The family Iflaviridae of insect viruses includes important pathogens of the western honeybee (Apis mellifera): deformed wing virus (DWV), sacbrood virus (SBV), and slow bee paralysis virus (SBPV). The icosahedral capsids of iflaviruses protect single-stranded RNA genomes that are about 10,000 nucleotides long and are polyadenylated at the 3′ end. Capsid proteins VP1, VP2, and VP0, originating from one polyprotein, form a protomer, 60 of which assemble into a pseudo-T = 3 icosahedral capsid. Subunits VP3 of DWV and SBPV have 160-residue-long C-terminal extensions, which fold into globular domains protruding from the virion surface.

The genome release of iflaviruses can be induced in vitro by exposing the particles to acidic pH. We show that acidic pH induces expansion of the RNA genome in the DWV particle, which, in turn, triggers the swelling and flower-like opening of its capsid. Native virions of DWV at neutral pH are uniform in size with a radius (the distance of the center of the mass of a pentamer from the center of the capsid) of 135 Å. The changes in the organization of the RNA genomes of DWV in acidic pH are connected to the radial expansion of the particles by 15 to 33% relative to the native virions at neutral pH. Pentamers of capsid protein protomers maintain a similar structure to that of the native virion, but the distances between the centers of masses of adjacent pentamers increase from 141 Å in the native virions to 164 to 192 Å in the expanded particles. In silico simulations of the expansion of DWV capsid have shown that residues 1 to 61 from the N termini of VP2 subunits can change their conformations and mediate attractive interpentamer interactions up to a distance of 7 nm. Therefore, the N termini of VP2 subunits enable the flexible expansion of DWV capsids and the deviation of its overall structure from icosahedral symmetry. The capsids of genome-containing particles being larger than those of empty particles provide evidence that at acidic pH, the genome exerts pressure on the inside of the capsid. After 30 min of incubation in phosphate-buffered saline (PBS) with pH 5.5 at 34°C, the capsids of 80% of DWV particles were open in a manner reminiscent of the opening of petals of a flower. The opening or removal of a single pentamer from the expanded DWV capsid results in the formation of a pore with a diameter of 190 Å, which is sufficient for the release of the RNA genome without major unwinding of its putative secondary and tertiary structure.

> GEESRNTTVLDTTTTLQSSGFGRAFFGEAFNDLKTLMRRYQLYGQLLLSVTTDKDIDHCMFTFPCLPQGLALDIGSAGSPHEIFNRCRDGIIPLIASGYRFYRGDLRYKIVFPSNVNSNIWVQHRPDRRLEGWSAAKIVNCDAVSTGQGVYNHGYASHIQITRVNNVIELEVPFYNATCYNYLQAFNASSAASSYAVSLGEISVGFQATSDDIASIVNKPVTIYYSIGDGMQFSQWVGYQPMMILDQLPAPVVRAVPE;> MDNPNPGPDGEGEVELEKDSNVVLTTQRDPSTSIPAPVSVKWSRWTSNDVVDDYATITSRWYQIAEFVWSKDDPFDKELARLILPRALLSSIEANSDAICDVPNTIPFKVHAYWRGDMEVRVQINSNKFQVGQLQATWYYSDHENLNISSKRSVYGFSQMDHALISASASNEAKLVIPFKHVYPFLPTRIVPDWTTGILDMGALNIRVIAPLRMSATGPTTCNVVVFIKLNNSEFTGTSSGKFYASQIRAKPE;> DNPSYQQSPRHFVPTGMHSLALGTNLVEPLHALRLDAAGTTQHPVGCAPDEDMTVSSIASRYGLIRRVQWKKDHAKGSLLLQLDADPFVEQRIEGTNPISLYWFAPVGVVSSMFMQWRGSLEYRFDIIASQFHTGRLIVGYVPGLTASLQLQMDYMKLKSSSYVVFDLQESNSFTFEVPYVSYRPWWVRKYGGNYLPSSTDAPSTLFMYVQVPLIPMEAVSDTIDINVYVRGGSSFEVCVPVQPSLGLNWNTDFILRNDEEYRAKTGYAPYYAGVWHSFNNSNSLVFRWGSASDQIAQWPTISVPRGELAFLRIKDGKQAAVGTQPWRTMVVWPSGHGYNIGIPTYNAERARQLAQHLYGGGSLTDEKAKQLFVPANQQGPGKVSNGNPVWEVMRAPLATQRAHIQDFEFIEAIPE> MEMVKSRSKVAIIGAGFVGASAAFTMALRQTANELVLIDVFKEKAIGEAMDINHGLPFMGQMSLYAGDYSDVKDCDVIVVTAGANRKPGETRLDLAKKNVMIAKEVTQNIMKYYNHGVILVVSNPVDIITYMIQKWSGLPVGKVIGSGTVLDSIRFRYLLSEKLGVDVKNVHGYIIGEHGDSQLPLWSCTHIAGKNINEYIDDPKCNFTEEDKKKIAEDVKTAGA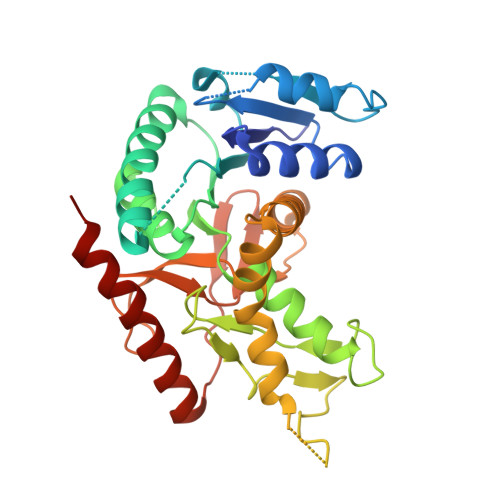TIIKNKGATYYGIAVSINTIVETLLKNQNTIRTVGTVINGMYGIEDVAISLPSIVNSEGVQEVLQFNLTPEEEEALRFSAEQVKKVLNEVKNL> SNAHGFHMPAEWEPHSQCWIGWPERADNWRDGAVHAQLVFTRVAAAISRFEKVTVCASSA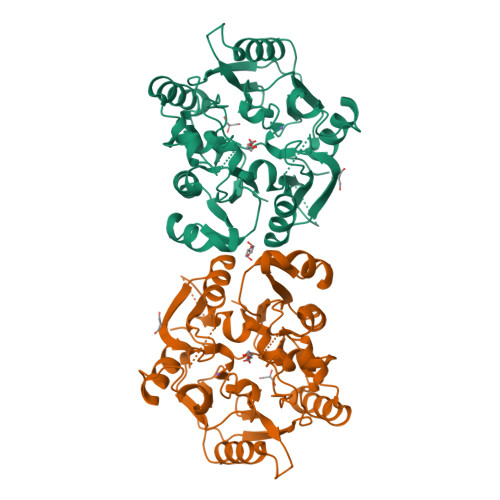QWENARNQLPDHVRVVEISSNDSWFRDIGPTFVVRRETSKSDDAEHRIAGIDWTFNSWGGLEDGCYCDWSLDSLVKKKILDVERIPRFSHSMVLEGGSIHVDGEGTCITTEECLLNKNRNPHLSKSQIEDELKAYLGVRKVIWLPRGLYGDDDTNGHVDNMCCFVRPGAVLLSWTDDKTDPQYERSEEAYSLFSSVTDANGRKFEVIKLHVPGPLYMTEKEAAGVFQDDGAKPRLPGTRLAASYVNFYIANGAIIAPQFGDKKWDDEAIRVLSKTFPHHEVVGIEGSREIVLSGGNIHCITQQQPAI>[4x]MLKQVEIFTDGSCLGNPGPGGYGAILRYRGREKTFSAGYTRTTNNRMALMAAIVALEALKEHCEVILSTDSQYVRQGITQWIHNWKARGWKTADKKPVKNVDLWQRLDAALGQHQIKWEW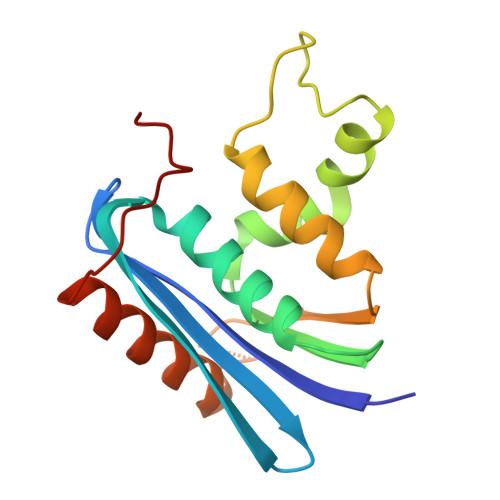VKGHAGHPENERCNELARAAAMNPTLEDTGYQVEV> MLFVLQCTAHTHTHTHTCRPQHLVAPLASLCRSLVVVSASLSPFHRPSLRVGHTVQCQARSHVSPLPTHLLFSSLALAACAHARRACRGAFSYLTATTITITVTTTFTTFFLFSVVLHPRFNGDRAAKAKTGKKMWRRSCCVLAPSIPRSVWDPAHYNENWVDSYSTSIADRRHWPAKKWSIGLEPRTPRDWLRFSYRNLAYAYNGALRACATFPEMLVYYKEMKQRGVKVDVDTLNALLSRAARYEHIQVDDVFLLFDELTALGARPDIASVETLHTVLEHAAHQPPEWRETRRRQLVELYQYLALEEIERLAPHRVDALLSAQIARLRGNLKQLNASLSPSVYRRYFAAIDLGETLIQEVHNFLWEYVGADHAAMDVPSLQLRIPFVASVMKRPLATADPAKVKATDFEDTDVCSVLLAAVERCVDGNFHDRRPVSERRMYLALLTMLTSSGVLYTADLMAQMMDVVKYSRDDRGRDRDAQRLLRYALRGSSAANDAAYRELWRAVAPPVDARVVGRYLASRDPWSPVHICYDRSFQFRAFPALQQITQSQCSSSSSSSSSSSTDAAAVAASTAAGAGSSSTAAAAAEPDEALEGVSAGPPPGTVAAKTAEALQQRWDDVRRLIDITGVLKPGAGLTSARTGSAAPTQEAAQQAMEVFTGAAAFLRGVATGCRYGELADALAIQAVGDGQQQHHHAPRATPLGGAAATAGAARSSSGNVNTELYAGGLDFDVWQRLMQCVQQLRQDMEQFMAQQYEAHGLQVEPEFECWEAMLVVLRCIL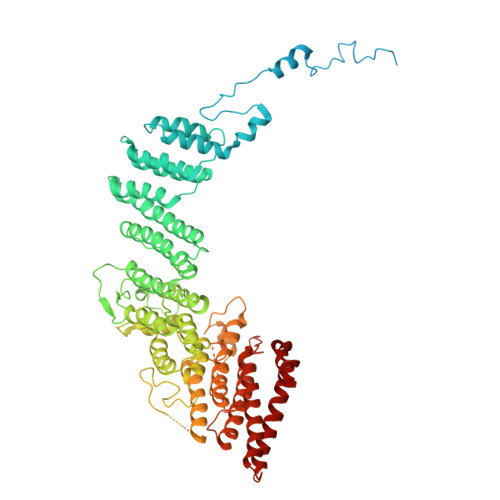DFCLVHTQQYGRTAGGGMAENLFLESAQLRAQLVEESRTRFNGRMRILWLQEV[[(2R,3S,4R,5R)-5-(6-aminopurin-9-yl)-3,4-bis(oxidanyl)oxolan-2-yl]methoxy-oxidanyl-phosphoryl] 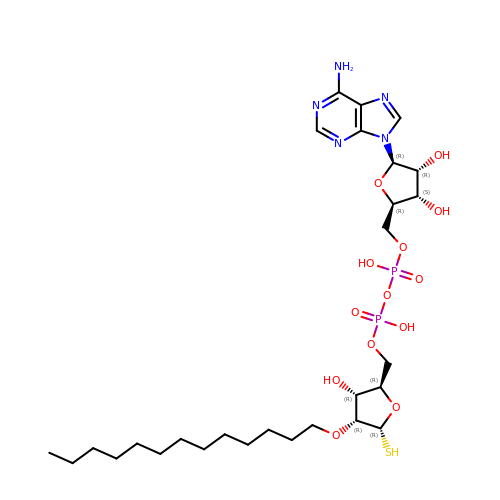[(2R,3R,4R,5R)-3-oxidanyl-5-sulfanyl-4-tridecoxy-oxolan-2-yl]methyl hydrogen phosphate | C28 H49 N5 O13 P2 S | VSVPTUFDWKYDGH-VBLNILRESA-N> HHHHHHGLIQERRSHEVNPAAHLTGANSSLTGSGGPLLWETQLGLAFLRGLSYHDGALVVTKAGYYYIYSKVQLGGVGCPLGLASTITHGLY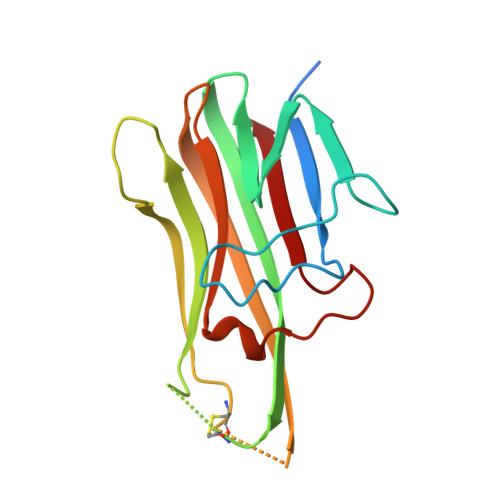KRTPRYPEELELLVSQQSPCGRATSSSRVWWDSSFLGGVVHLEAGEEVVVRVLDERLVRLRDGTRSYFGAFMV>[4x]GAMGSMTDDKDVLRDVWFGRIPTCFTLYQDEITEREAEPYYLLLPRVSYLTLVTDKVKKHFQKVMRQEDISEIWFEYEGTPLKWHYPIGLLFDLLASSSALPWNITVHFKSFPEKDLLHCPSKDAIDAHFMSCMKEADALKHKSQVINEMQKKDHKQLWMGLQNDRFDQFWAINRKLMEYPAEENGFRYIPFRIYQTTTERPFIQKLFRPVAADGQLHTLGDLLKEVCPSAIDPEDGEKKNQVMIHGIEPMLETPLQWLSEHLSYPDNFLHISIIPQPTD;>GSMSSGLRAADFPRWKRHISEQLRRRDRLQRQAFEEIILQYNKLLEKSDLHSVLAQKLQAEKHDVPNRHEI[4x]

Macroautophagy, referred to hereafter as autophagy, is a cellular process by which proteins and organelles are degraded and recycled through sequestration within autophagosomes and delivery to lysosomes. ATG5 plays a role in elongation of the phagophore and its subsequent maturation into the complete autophagosome. ATG12 is a ubiquitin-like protein that covalently binds ATG5, and this conjugate noncovalently binds ATG16L1. The ATG12–ATG5-ATG16L1 complex functions in part as an E3 ligase to facilitate the conjugation of LC3 to phosphatidylethanolamine, generating LC3-II.

Whole exome sequencing identified a homozygous missense mutation, hg19 chr6:106,727,648 T>A, corresponding to E122D in ATG5 as the only damaging mutation within the genetically identified chromosomal linkage interval. Crystal structure of the resulting ATG12–ATG5-ATG16L1 complex indicated that E122 is located in the vicinity of the ATG12–ATG5 interaction surface; hence, we predicted that the mutation in ATG5 could affect the conjugation of ATG12. We could detect the ATG12–ATG5 complex when both wild-type proteins were co-expressed, but we could only detect a minimal amount of the ATG12–ATG5E122D complex. Interestingly, expression levels of ATG5WT and ATG5E122D monomers were comparable to each other, indicating that the mutation affects the conjugation process, rather than the stability of proteins. To confirm that the mutation does not overtly alter the structure of ATG5 or binding to ATG16L1, we analyzed formation of the noncovalent ATG5-ATG16L1 complex using constructs containing a TEV protease site. Both wild-type and mutant ATG5 protein were efficiently co-precipitated with ATG16L1. Indeed, the co-crystal structure of a human ATG5E122D-ATG16L1 complex superimposes well with the previously determined structure of the WT proteins, with the major obvious difference being replacement of the side-chain. Although the overall structure of the E122D mutant ATG5 superimposes well with the wild-type protein, the mutation causes a striking decrease in the level of ATG12–ATG5 conjugate that is formed when the C terminus of ATG12 is covalently linked to Lys130 of ATG5. We speculate that the E122D mutation causes subtle changes in the conformational dynamics that propagate to Lys130, which is less than 10 Å away, resulting in less ATG12–ATG5, which in turn leads to reduced LC3/Atg8 conjugation. Our results indicate that E122D is a partial loss-of-function allele that impairs but does not completely abolish ATG5 activity.> SNFSGFTKGTDIADLDAVAQTL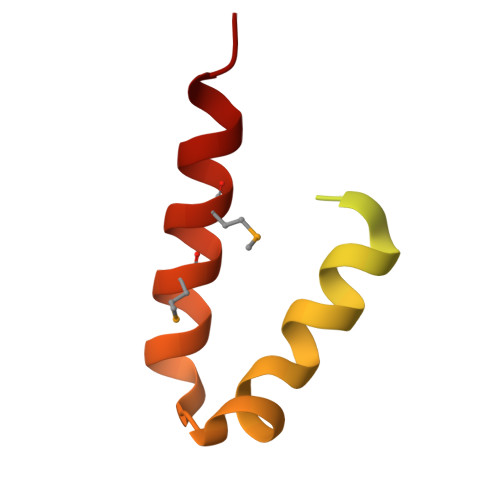KKPADDANKAVNDSIAALKDKPDNPALLADLQHSINKWSVIYNINSTIVRSMKDLMQGILQKFP> GSHMMTSSTAVPANPSADNSAKKVYQWLNGLPDSNGKKLISGIFGGYSNIGGDSGFSLAQGNAIKDATGKFPAIYGADYARGWDVSAPGDEASLIDHSCNSDLISHWKNGGLVAISHHLPNPFYAGNNPGTGEGGLKKAISNDEFATILQDGTGARQRWLSLLDKVAEGLQELRDNGVPVLYRPLHEMNGEWFWWGATGYNTNDATRQDLYRRLYQDVFSYFVN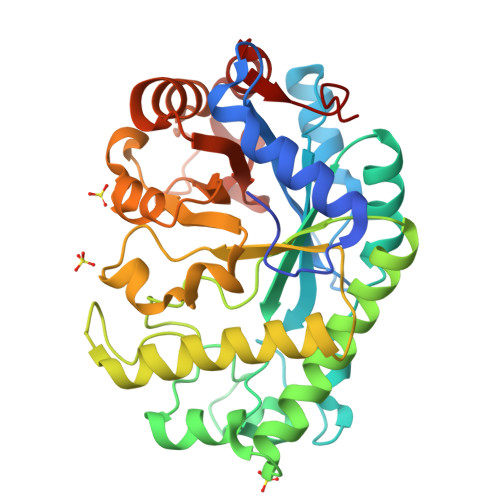TKGLTNLLWVFSPDANRDHKTAYYPGAGYVDIAGLDFYTDNPASLSGYDEMLGLNKPFGLVEVGPSTTNGQYDYAVLVNTILQNFPKTIMFVPWNDGWSPVKNQNAAAAFNNGSVINLGDISISW>[2x]MYEAIGHRVEDGVAEITIKLPRHRNALSVKAMQEVTDALNRAEEDDSVGAVMITGAEDAFCAGFYLREIPLDKGVAGVRDHFRIAALWWHQMIHKIIRVKRPVLAAINGVAAGGGLGISLASDMAICADSAKFVCAWHTIGIGNDTATSYSLARIVGMRRAMELMLTNRTLYPEEAKDWGLVSRVYPKDEFREVAWKVARELAAAPTHLQVMAKERFHAGWMQPVEECTEFEIQNVIASVTHPHFMPCLTRFLDGHRADRPQVELPAGV;> MYEAIGHRVEDGVAEITIKLPRHRNALSVKAMQEVTD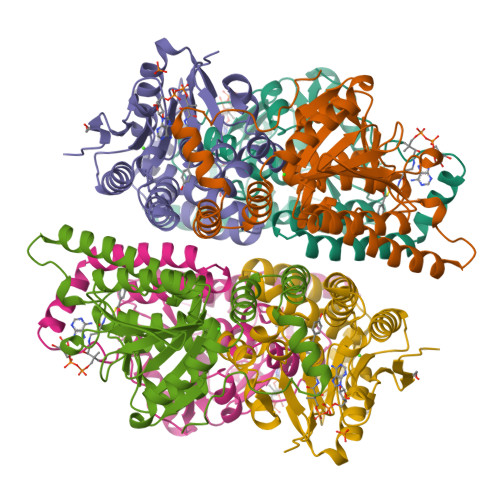ALNRAEEDDSVGAVMITGAEDAFCAGFYLREIPLDKGVAGVRDHFRIAALWWHQMIHKIIRVKRPVLAAINGVAAGGGLGISLASDMAICADSAKFVCAWHTIGIGNDTATSYSLARIVGMRRAMELMLTDRTLYPEEAKDWGLVSRVYPKDEFREVAWKVARELAAAPTHLQVMAKERFHAGWMQPVEECTEFEIQNVIASVTHPHFMPCLTRFLDGHRADRPQVELPAGV>[2x]MQNPQNLIWIALEMTGLDPDRDVIIEMATIVTDSDLNTLAEGPVIAIHQPEEILAGMDEWNTRQHGQSGLTQRVRESTVSMAEAEAQTLAFLEQWVPK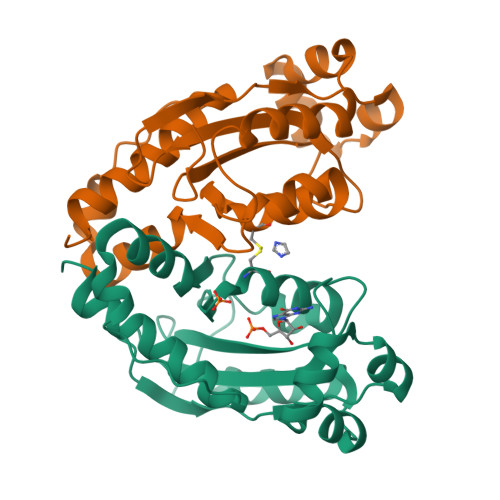RSSPICGNSICQDRRFLYRHMPRLEGYFHYRNLDVSTLKELAARWAPQVRESFKKGNTHLALDDIRESIAELRHYRDHFIKL(2R)-N-[(4M)-4-(4-amino-7-methyl-7H-pyrrolo[2,3-d]pyrimidin-5-yl)-3-methylphenyl]-2-(3-fluorophenyl)-2-hydroxyacetamide 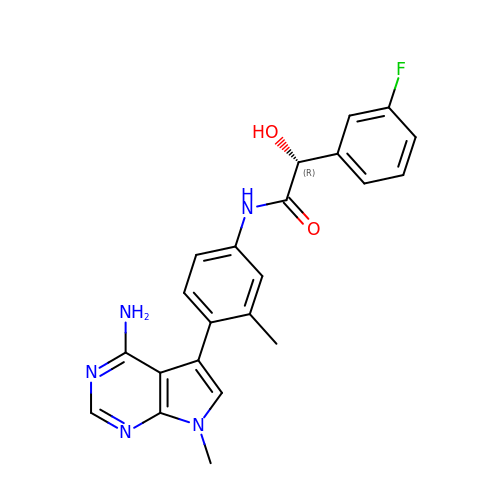| C22 H20 F N5 O2 | HLLGQFADOTVZQN-LJQANCHMSA-N>DKATIPSESPFAAAEVADGAIVVDIAKMKYETPELHVKVGDTVTWINREAMPHNVHFVAGVLGEAALKGPMMKKEQAYSLTFTEAGTYDYHCTFHP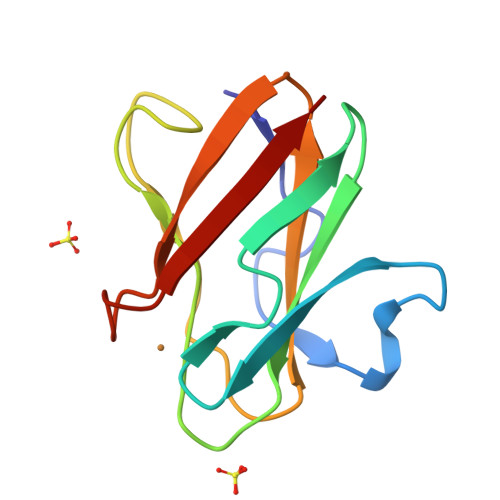FMRGKVVVE[2x]>GSHMKHTEL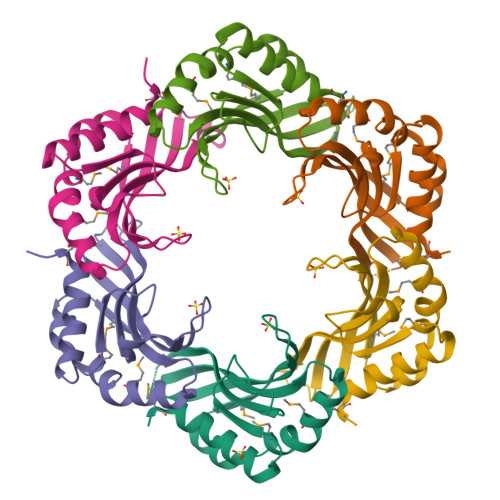RAAVLDALEKHDTGATFFDGRPAVFDEADFPAVAVYLTGAEYTGEELDSDTWQAELHIEVFLPAQVPASELDAWMESRIYPVMSDIPALSDLITSMVASGYDYRRDDDAGLWSSADLTYVITYEM[12x]>KESAAAKFERQHMDSGNSPSSSSNYCNLMMCCRKMTQGKCKPVNTFVHESLADVKAVCSQKKVTCKNGQTNCYQSKSTM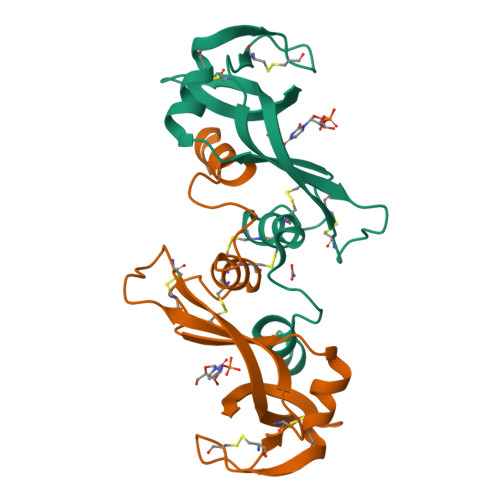RITDCRETGSSKYPNCAYKTTQVEKHIIVACGGKPSVPVHFDASV[2x]> HAEGTFTS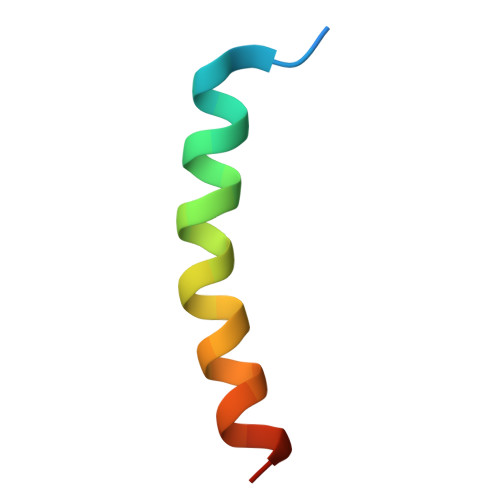DVSSYLEGQAAKEFIAWLVKGRG4-nitrophenyl beta-D-glucopyranosyl-(1->4)-beta-D-glucopyranosyl-(1->4)-beta-D-glucopyranoside | C24 H35 N O18 | 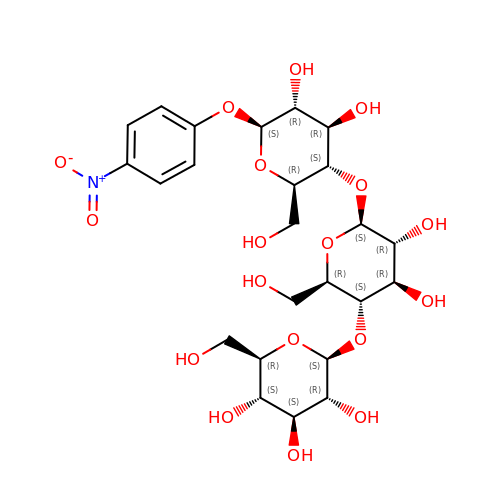BETIRLUWOMCBBJ-ZENQEEDISA-N In this work, we exhaustively probe the ability of all 36 immobile HJ sequences to form DNA crystals in two different designed systems. Three separate self-assembling DNA crystal systems are described in this report: the “4 × 5” and “4 × 6” designs (collectively referred to as the 4 × N systems), and a third construct with a “scrambled” sequence variant of the 4 × 6 lattices. Self-assembly was mediated by three constituent oligonucleotides: (S1) containing four sequence repeats of either 5 or 6 bases; (S2) composed of 21 bases containing complementary regions to both (S1); and (S3) which forms the second junction crossover. The HJ serves as the fundamental component at the core of each unit, and the ultimate assembly of the full lattice is facilitated by the complementary 2-base sticky ends that tail each duplex.

Each asymmetric unit could be defined as either a HJ containing 10 and 11 bp on each arm, or as a 21-bp linear duplex. We hypothesized that it might be possible to introduce other unique immobile sequences that could provide slight perturbations in the junction angle, to potentially reduce the strain in the original system and yield a “relaxed,” periodic lattice. The 4 × 5 system robustly crystallized with 75% of the junctions, and we obtained crystals in all but 9 of 36 sequences. Of the resulting structures, 18 exhibited P32 symmetry with average cell dimensions a = b = 68.85 Å c = 60.09 Å, with only nine retaining the original P3221 symmetry with average cell edges a = b = 68.17 Å c = 60.60 Å. Although the cell parameters between the two symmetries were virtually indistinguishable, the differences between the periodicity of the lattices is dramatic, with vastly different cavity sizes. While the highest resolution achieved for the J1 system was 3.1 Å, in roughly half of the crystals measured the resolutions were 3.05 Å or better, and as high as 2.9 Å (J6) and 2.75 Å (J19), for the P32 and P3221 symmetries, respectively. The mean angles across all junctions within the groups were 56.05° (σ = 1.63) and 56.59° (σ = 1.50) for the P32 and P3221, respectively. We hypothesize that even a small difference in junction angles could have a significant global effect on the assembly of the lattice, thereby eliminating the strain in the P3221 lattices.

> GAGCAGACCAGACGCCACTCA;> CGTCT;> TCTGAGTGG;> GGTCTGC> AGAGCGUUGCGUCCGAAAGUCGCC;> GCGACACGGCUCUUUAAAAACAAAAGGAGA

We present crystal structures of a new NAD+-binding riboswitch termed NAD+-II, bound to nicotinamide mononucleotide (NMN), nicotinamide adenine dinucleotide (NAD+) and nicotinamide riboside (NR). The RNA structure comprises a number of structural features including three helices, one of which forms a triple helix by interacting with an A5 strand in its minor-groove, and another formed from a long-range pseudoknot. Unusually the riboswitch binds two molecules of ligand, bound at distinct, non-overlapping sites in the RNA. Binding occurs primarily through the nicotinamide moiety of each ligand, held by specific hydrogen bonding and stacking interactions with the pyridyl ring.

The first comprised two strands made by chemical synthesis, so that the terminal loop of helix P1a was not present. 5-Bromocytidine was incorporated at C21 in order to determine the phases by SAD. The two-strand form of the riboswitch bound to NMN crystallised in space group P3221 and diffracted to a resolution of 2.23 Å; these data were used to determine the structure by Br-SAD. In the complete riboswitch P1a is a stem loop, but in our construct the loop is not present.>[4x]MPYDHNAEADFAASEVARMLVADPGLCYDAASLPASISASASYEPSAAGWPKADGLVSVLEGGTSTQRAIALEYKRPQEGIHGLLTAIGQAHGYLHKGYSGAAIVIPGRYSSHPTPAEYVRDVLNAISGSRAIAVFSYSPPDTTSPTPFAGRIQCVRPLVFDAGRVHLRPANQGPKTQWVHMREGSTTRDAFFRFLQVAKRLSADPTAPRPTLRSELVAAIGRLAPGRDPIEYITNTADNKFLTKVWQFFWLEWLATPAVLTPWKLEAGVYSAPGARTRILREDGTDFSQLWEGRVNSLKETIAGMLNRGEISEAQGWEAFVGGISATGGGQDKQGVRARAHSYREDIDSALAQLRWIEDDGLPTDQGYRFMTICERYGGANSRAAIDYMGATLIQTGRYASFLHYINRLSERKFAENPLAYTKPGPGGMPVFTEESYWEYLQDLETKLTDELRVMRKVSGRARPRVRTTFQVELTLLRNYGFVSSTRHRLGVGIPIDWEQVVQALNVDL

Type IIS restriction endonucleases (the topic of this study) combine independently folded target recognition (‘TRD’) and endonuclease (‘EN’) domains within a single protein chain, cleaving DNA at one or both sides of their target site. Here, we report biochemical analyses and high-resolution crystallographic and CryoEM structures (in the presence and absence of bound DNA) of the Type IIS REase PaqCI. It forms a tetramer in solution in both the absence and presence of bound DNA, recognizes a longer target than FokI (5′-CACCTGC-3′), and cleaves each strand of bound DNA much closer to the bound target site (4 and 8 bases downstream, respectively). The enzyme displays a similar tetrameric organization of target recognition domains in the absence or presence of bound substrate, with a significant repositioning of endonuclease domains in a trapped DNA-bound complex that is poised to deliver the first of a series of double-strand breaks.

A 50 bp double-stranded DNA construct containing the enzyme's target site and sufficient downstream duplex to extend past the enzyme's cleavage site was used to generate a DNA-bound enzyme complex in the presence of calcium (which facilitates the formation of a productive cleavage complex but inhibits cleavage). A CryoEM density map of the DNA-bound enzyme, corresponding to approximately 3.0–3.6 Å resolution, was generated from 1,291 micrographs and over 800 000 particles. All four TRDs within the PaqCI tetramer are individually engaged with four corresponding double-stranded DNA duplexes through contacts with the enzyme's target site sequence to form a complex to cleave a single DNA duplex. The binding of DNA imparts minimal rearrangement of the TRD tetrameric assembly. In the DNA-bound complex, all four endonuclease domains (ENs) have dissociated from their original positions, where they were originally sequestered against their corresponding target recognition domains (TRDs). Two of the ENs, extending from one of the two enzyme dimers in the protein tetramer, have reformed a catalytic EN dimer around the cleavage site of one of the bound DNA duplexes (indicated by boxes in all panels of Figure 4 and in Figure 6). The other EN domain (colored green) is engaged with the opposing strand of the same cleavage site in trans (i.e. that domain extends across the dimer interface from a TRD bound to a different DNA duplex and target site). The cis-acting EN domain is positioned appropriately for cleavage of the phosphodiester located 4 bp from the target site, while the trans-acting EN domain (which has moved a much longer distance to re-establish contact with its partner) is positioned appropriately to cleave the phosphodiester bond 8 bp from the target site on the opposing strand. The opposing two EN domains (also previously packed against their own TRDs in the DNA-free apo-enzyme), which are also released from their TRDs as a result of DNA binding, are unobservable and appear to be disordered.>[4x]MTVPLYKQIASLIEDSIVDGTLSIDQRVPSTNELAAFHRINPATARNGLTLLVEAGILYKKR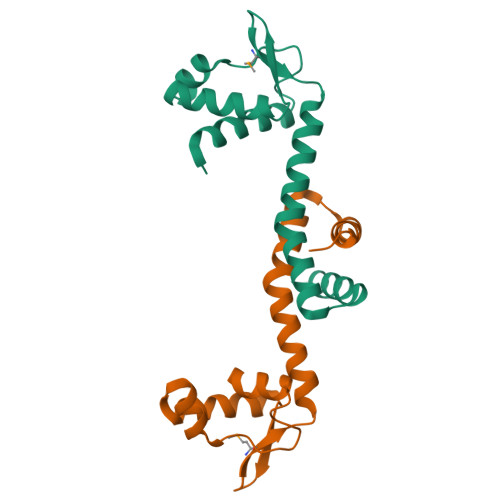GIGMFVSAQAPALIRERRDAAFAATYVAPLIDESIHLGFTRARIHALLDQVAESRGLYKLEHHHHHH> MADADPDVLKVALLPDENASELIKRNQPLKDYLEEHLDKKVQLIVTTDYSSMIEAMRFGRIDLAYFGPLSYVMAKSKSDIEPFAAMVIDGKPTYRSVIIANVASGVNEYADLKGKRMAYGDRASTSSHLIPKTVLLETADLTGGQDYEQHFVGTHDAVAVNVANGNADAGGLSEVIFNHAAERGLIDPSKVKVLGYSGEYPQYPWAMRSNLSPELKTKVRDVFVGIDDPEVLRNFKAEAFAPITDADYDVIRNMGSLLGLDFATMLEHHHHHH

Here we elucidate the molecular basis of high-affinity phosphite and hypophosphite acquisition by determining the ligand-binding affinity and structure of the PBPs of phosphite and hypophosphite ABC transporters from environmental microorganisms. We over-produced and purified PBPs of three putative phosphite transporters; PtxB from the globally important marine diazotroph Trichodesmium erythraeum IMS101 (Te_PtxB), PhnD from the oceanic picocyanobacteria Prochlorococcus marinus MIT9301 (Pm_PhnD)35 and PtxB from the soil bacterium Pseudomonas stutzeri WM88 (Ps_PtxB), as well as a PBP from a putative hypophosphite transporter, HtxB, also from P. stutzeri WM88 (HtxB)18. The structures reveal that ligand specificity, measured here by thermophoresis, arises from a combination of steric considerations and the interaction between a ligand P-H hydrogen atom and an aromatic π system in the binding pocket. The structures of two distinct types of phosphite-binding protein and a hypophosphite-binding protein reveal that a P-H…π interaction ensures high-affinity binding of specific ligands, representing a universal mechanism in these PBPs for recognising ligands with a P-H bond.

We also obtained structures of phosphite and MPn complexed Ps_PtxB and determined the associated ligand affinities; both the structures and binding data were similar to the other phosphite-binding proteins discussed previously. Analysis of the conformational change between the open and closed, phosphite-bound structure of Ps_PtxB using DynDom42 revealed that domain closure is induced by a ~60° rotation around an axis that lies between the two lobes. This is facilitated by flexible loops that form the hinge region between the lobes (residues A85-T93 and Y200-Q202), as well as residues from the extreme end of the C-terminal helix (G255-L258). Superposition of the individual lobes of Ps_PtxB in the open and closed conformations shows that lobe 2 (residues 96–196, 0.35 Å RMSD cα) adopts a very similar structure, with the conserved STS-H motif (S124, T125, S126 and H155) spatially conserved in both conformations. The positions of Y94, which hydrogen bonds to one of the phosphite oxygen atoms in the closed structure, and D16, which hydrogen bonds to and stabilises the capping tyrosine in the closed structure, move ~7 Å and ~4.5 Å (cα-cα), respectively, on ligand binding. Y94 resides on the hinge region, the conformation of which alters substantially during domain closure, whilst D16 sits on a flexible loop that latches over the binding pocket in the closed conformation. In addition, the B-factors of the core residues in lobe 2 are much lower in the closed, ligand bound, conformation compared to those in the open structure, implying lower overall flexibility when phosphite is bound to the protein.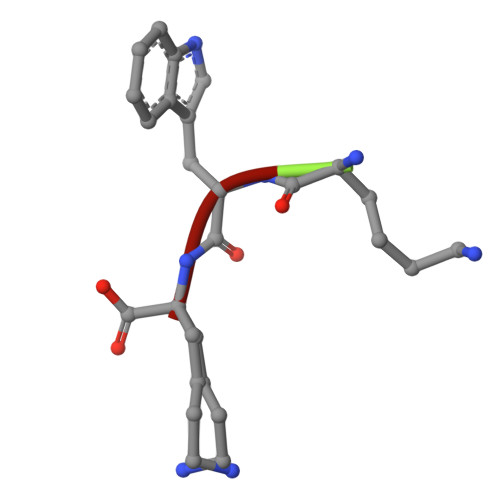> KWK>[2x]MTERIRNVALRSKVCPAETASELIKHGDVVGTSGFTGAGYPKEVPKALAQRMEAAHDRGEKYQISLITGASTGPQLDGELAKANGVYFRSPFNTDATMRNRINAGETEYFDNHLGQVAGRAVQGNYGKFNIALVEATAITEDGGIVPTSSVGNSQTFLNLAEKVIIEVNEWQNPMLEGIHDIWDGNVSGVPTRDIVPIVRADQRVGGPVLRVNPDKIAAIVRTNDRDRNAPFAAPDETAKAIAGYLLDFFGHEVKQNRLPPSLLPLQSGVGNVANAVLEGLKEGPFENLVGYSEVIQDGMLAMLDSGRMRIASASSFSLSPEAAEEINNRMDFFRSKIILRQQDVSNSPGIIRRLGCIAMNGMIEADIYGNVNSTRVMGSKMMNGIGGSGDFARSSYLSIFLSPSTAKGGKISAIVPMAAHVDHIMQDAQIFVTEQGLADLRGLSPVQRAREIISKCAHPDYRPMLQDYFDRALKNSFGKHTPHLLTEALSWHQRFIDTGTMLPSSLEHHHHHH

Acetobacter aceti strain 1023 and other acetic acid bacteria use succinyl-CoA:acetate CoA-transferase (AarC) in a variant citric acid cycle that is required for a robust acetic acid resistance (aar) phenotype. Strong selection for key roles in acetic acid resistance and central metabolism appear to have optimized the structural and functional properties of AarC, making it an excellent representative of the class I CoA-transferase superfamily. Class I acyl-CoA:carboxylate CoA-transferases produce reactive acylglutamyl anhydride intermediates that acylate CoA, forming either an acyl-CoA product and a free enzyme or a protein glutamyl-CoA thioester and a carboxylate product. A closed active site enables AarC to engage, immobilize, and desolvate acyl-CoA substrates and to stabilize covalent adducts of Glu294.

The AcCoA ketone analog 1a, in which the thioester sulfur atom is replaced by a methylene group, was tested for its ability to form a hemiacetal analog of the tetrahedral hemithioacetal intermediate stabilized by the external oxyanion hole. Compound 1a was unexpectedly degraded by microbial contamination, yielding a crystal containing an acetylglutamyl anhydride adduct and a CoA analog (modeled as 2a). Despite our expectations, electron density for Glu294A was most consistent with a mixture composed of both free carboxylate and acetylglutamyl anhydride adduct in a 0.4/0.6 ratio, with a relatively narrow range of B-factors. Since density associated with the 3′-phosphate was ambiguous and weak, the large ligand in subunit A was modeled as 2b. The electron density associated with the large ligand in subunit B did not extend beyond carbon atom C3P, so it was modeled as 3′-phosphoadenosine 5′-(O-(N-methyl-R-pantothenamide))pyrophosphate. An active site acetate ligand was also included in subunit B. Subunit A (5e5hA) adopted an open conformation distinctly different from a partially closed conformation observed for an AcCoA-derived acetylglutamyl anhydride (PDB entry 4eu6A). Subunit B (5e5hB) adopted a partially closed conformation similar to that observed for the glutamyl-CoA thioester adduct bound to acetate (PDB entry 4eu6B), even though 1a and truncated derivatives (e.g., 2a and 4a) cannot form thioesters. A more likely explanation for the difference is the absence of an acetylglutamyl anhydride from the AarC•2a crystals; crystals obtained from AarC+1a adopt an intermediate conformation characteristic of other covalent adducts (lower right quadrant) that may protect the labile anhydride. Degradation of an AcCoA analog by unidentified microbial enzymes produced an activated acetyl donor and acetate, which suggests that ester analogs of AcCoA (e.g., 5a) could be used to produce a stabilized acetylglutamyl anhydride on AarC.1-[(2-chlorophenyl)methyl]pyrrole-2-carboxamide | C12 H11 Cl N2 O | 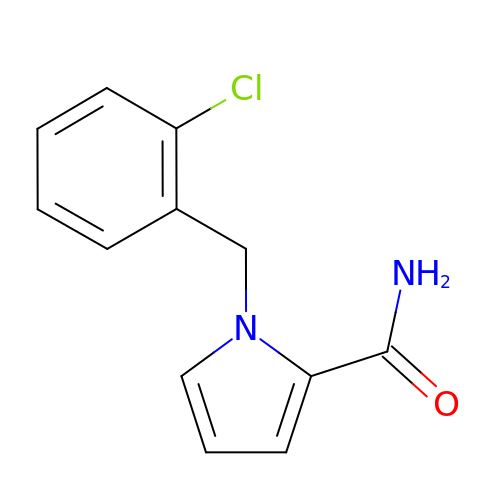FNWQVYIDFQBAEE-UHFFFAOYSA-N> QSACTLQSETHPPLTWQKCSSGGTCTQQTGSVVIDANWRWTHATNSSTNCYDGNTWSSTLCPDNETCAKNCCLDGAAYASTYGVTTSGNSLSIDFVTQSAQKNVGARLYLMASDTTYQEFTLLGNEFSFDVDVSQLPCGLNGALYFVSMDADGGVSKYPTNT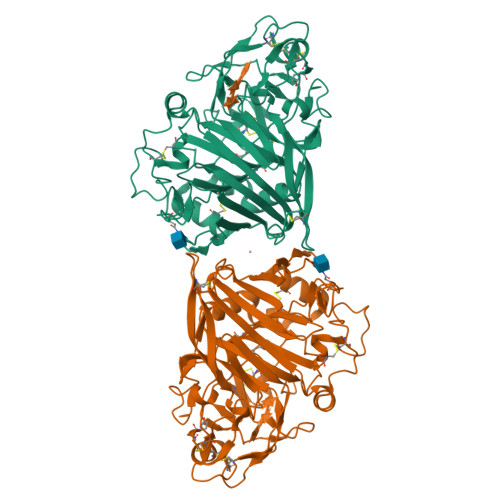AGAKYGTGYCDSQCPRDLKFINGQANVEGWEPSSNNANTGIGGHGSCCSEMDIWQANSISEALTPHPCTTVGQEICEGDGCGGTYSDNRYGGTCDPDGCDWNPYRLGNTSFYGPGSSFTLDTTKKLTVVTQFETSGAINRYYVQNGVTFQQPNAELGSYSGNELNDDYCTAEEAEFGGSSFSDKGGLTQFKKATSGGMVLVMSLWDDYYANMLWLDSTYPTNETSSTPGAVRGSCSTSSGVPAQVESQSPNAKVTFSNIKFGPIGSTGNPSG>GPGS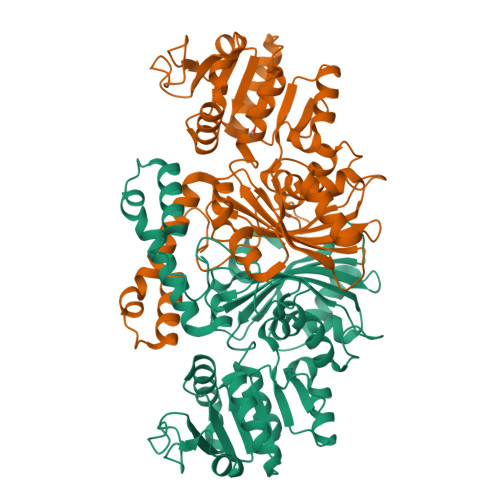MNVGLVGWRGMVGSVLMQRMQEEGDFDLIEPVFFSTSNAGGKAPSFAKNETTLKDATSIDDLKKCDVIITCQGGDYTNDVFPKLRAAGWNGYWIDAASSLRMKDDAVIILDPVNLNVIKDALVNGTKNFIGGNCTVSLMLMALGGLFRENLVDWMTAMTYQAASGAGAQNMRELLAQMGTLNGAVAAQLADPASAILDIDRRVLAAMNGDAMPTSQFGVPLAGSLIPWIDKDLGNGMSREEWKGGAETNKILGKPAMGEPGSVPVDGLCVRIGAMRCHSQALTIKLKKDVPLDEINGILASANDWVKVVPNEREASMRDLSPAKVTGTLSVPVGRLRKLAMGGEYLSAFTVGDQLLWGAAEPLRRMLRILLDK[2x]> CPTLDDTARGAYPIDSSQTYRIARLCLQPTTFLVKENGEFVPTKLVTRETTSLDQIQGELKVNSDGSLTFVEEDGIDFQPVTVQMAGGERIPLLFTVKNLVASTQPNVTSITTSTDFKGEFNVNGTKGQISLNVAKVDGRTGEIAGTFESEQLSNG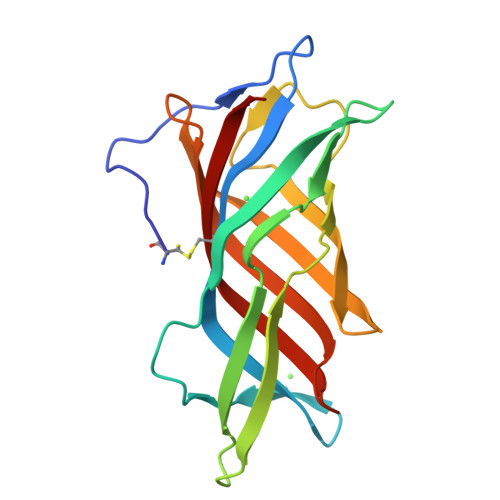HEVKIQGVFYASIEPA> DVYQEPTDPKFPQQWYLSGVTQRDLNVKAAWAQGYTGHGIVVSILDDGIEKNHPDLAGNYDPGASFDVNDQDPDPQPRYTQMNDNRHGTRCAGEVAAVANNGVCGVGVAYNARIGGVRMLDGEVTDAVEARSLGLNPNHIHIYSASWGPEDDGKTVDGPARLAEEAFFRGVSQGRGGLGSIFVWASGNGGREHDSCNCDGYTNSIYTLSISSATQFGNVPWYSEACS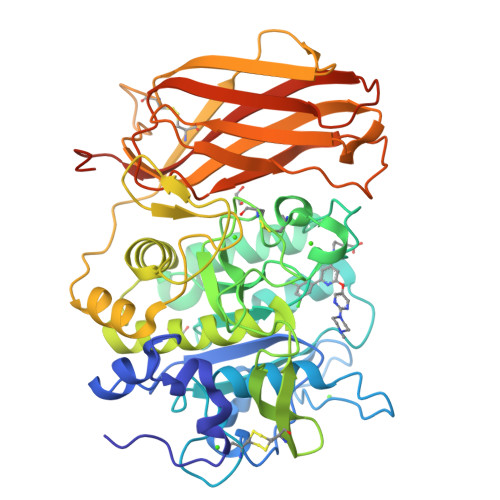STLATTYSSGNQNEKQIVTTDLRQKCTESHTGTSASAPLAAGIIALTLEANKDLTWRDMQHLVVQTSKPAHLNANDWATNGVGRKVSHSYGYGLLDAGAMVALAQDWTTVAPQRKCIIDILTEPKDIGKRLEVRKTVTACLGEPNHITRLEHAQARLTLSYNRRGDLAIHLVSPMGTRSTLLAARPHDYSADGFNDWAFMTTHSWDEDPSGEWVLEIENTSEANNYGTLTKFTLVLYGTAGENLYFQGDYKDDDDKGHHHHHH>GSHMTGGSVHSSPAIGQDGTIYVGSNDHYLYAINPNGKLKWKFETGGSVHSSPAIGQDGTIYVGSNDHYLYAINPNG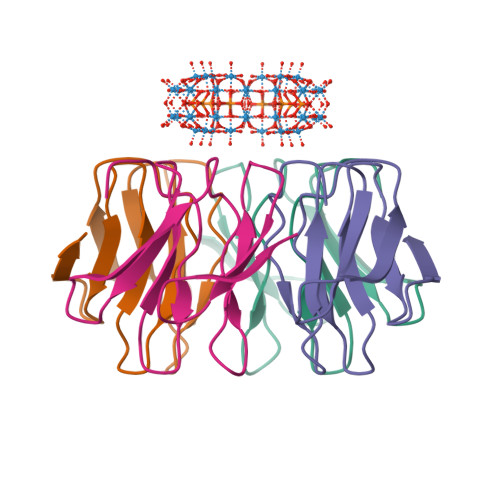KLKWKFE[4x]1,5-DI(4-AMIDINOPHENOXY)-3-OXA-PENTANE | C18 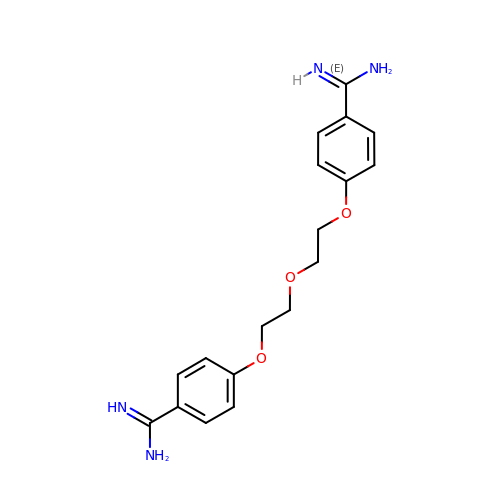H22 N4 O3 | RUGJWTYDBUIXNX-UHFFFAOYSA-N>[9x]MAHIFVKPELVAEIGVKQLQREIVLPGLVWTNPLTDFGGSKNDTITVRVPAITTANRRDLRDPDRTVIASELVEHSFGVTLDKHVYAALKFTDEQRTLDIRDYTKQVLMPQVSAVAYELEDYIAELIEGAPYEETIL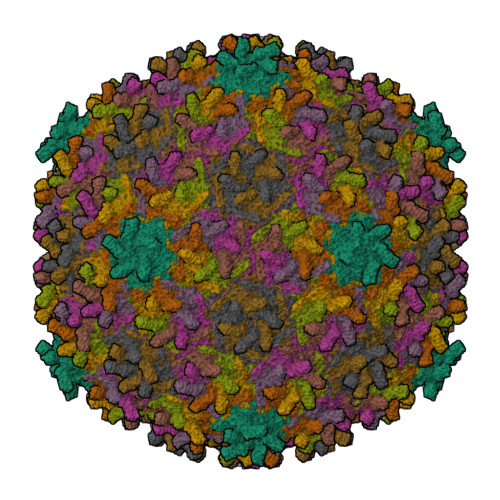IDPADTVPAFITADQRMGEANVPTDSRRLVVGSAVAAALAKDKQFRHADWSGDQANAALREAHVGRLAGMNVIRSNAIAPDKAYLWHRTAFILAYRTPVVPEGAKAGASFSANGVALRWLADYDYSQLGDRTLLDVFTGRKVVTEVDGSFVRAVELQLQASSITIVGGAFALATTTGTKQLKVRDDNGTDVTARCTFASSAGTKATVSAAGLVTGVAAGTADITASYVPPQGGTAKTATVTVTVP> SFVKDFKPQALGDTNLFKPIKI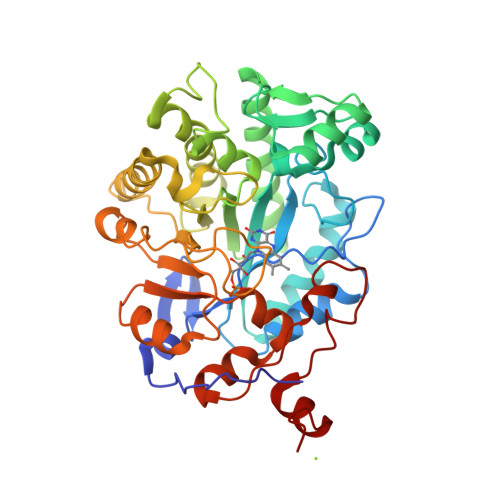GNNELLHRAVIPPLTRMRALHPGNIPNRDWAVEYYTQRAQRPGTMIITEGAFISPQAGGYDNAPGVWSEEQMVEWTKIFNAIHEKKSFVWVNLWVLGWAAFPDNLARDGLRYDSASDNVFMDAEQEAKAKKANNPQHSLTKDEIKQYIKEYVQAAKNSIAAGADGVEIHSANGYLLNQFLDPHSNTRTDEYGGSIENRARFTLEVVDALVEAIGHEKVGLRLSPYGVFNSMSGGAETGIVAQYAYVAGELEKRAKAGKRLAFVHLVEPRVTNPFLTEGEGEYEGGSNDFVYSIWKGPVIRAGNFALHPEVVREEVKDKRTLIGYGRFFISNPDLVDRLEKGLPLNKYDRDTFYQMSAHGYIDYPTYEEALKLGWDKK>GPLGSVREEIESLVQDSLMEMVKGVKNTIESDLASKKG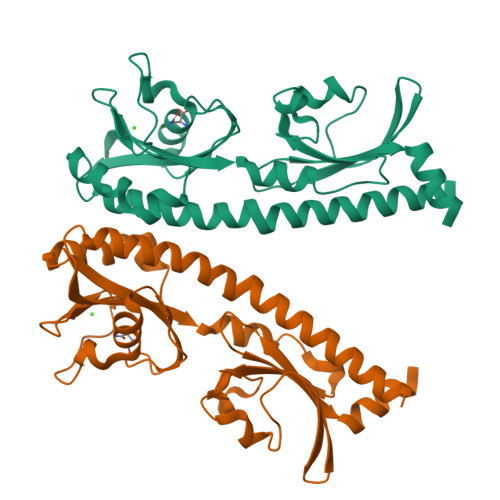LAQSTTEILQLDPTNKAFAKSVLESPNLKGSFLAIGLGYESDATVVENDDGWEPNADYDPRKRPWYVDAKRERKLVVTEPYVDISTKKIIISIGTPVYQQSNFVGAMFYDVELTQLAQLVNSVNLFDAGYLFITTKDGVTIAHPNAENNGEKFSQFLPNVDLKEGTQRIELDGKYYLVKFAQVPSESWYIGAVVDESIAFAMVDDLRHSSLIHHHHHH[4x]>MQLWDINDHPYLNIKGRFQRDENGDEVWVVSAKRMWSLTQNEWLSADEVEIFDDPLYAGEPGFSAMIHDHEFAIHKHCTDVVVSGKARAYAKRPVEQMECRLLLDGHIDKTLVIHGQRDWIEHGGSITVSNPQSFIDCDIDYSHAIGGEDERNRIGGGVASSNKVLLTQRVPSVFYPKEDWDATSKKVRVAGFGPIPPFFKQRYQLAGTFDDNWLENRRPLLPVDFDRRYYQSAPLDQQCKGYLQGGERLMLSGFSHDDIFSFRLPREKYRASADFGDDQEFKDLELYTVFVDTEKGVVSLTYSAAFACQEKEHLLKSTSIQAVVENTNERGLNNEKLEHHHHHH[2x]

Type VI secretion systems (T6SSs) are dynamic protein nanomachines found in Gram-negative bacteria that deliver toxic effector proteins into target cells in a contact-dependent manner. Prior to secretion, many T6SS effector proteins require chaperones and/or accessory proteins for proper loading onto the structural components of the T6SS apparatus. Next, we present both genetic and biochemical evidence that PIPY domains require a cognate DUF2169 protein to form a functional T6SS spike complex with VgrG. Based on these findings, we propose a model whereby DUF2169 proteins function as molecular chaperones that maintain VgrG–PIPY spike complexes in a secretion-competent state prior to their export by the T6SS apparatus.

To circumvent this obstacle, we next screened a panel of DUF2169 proteins encoded by other Vibrio spp. that are closely related to V. parahaemolyticus and found that the DUF2169 protein from Vibrio xiamenensis, which shares 64% pairwise sequence identity with DUF2169 from V. parahaemolyticus, readily crystallized and we were able to solve its X-ray crystal structure to a resolution of 1.85 Å. The resulting electron density was of excellent quality, and we were able to model the majority of the 337 amino acid protein except for its three N-terminal and 12 C-terminal residues. The overall structure of V. xiamenensis DUF2169 reveals that its secondary structure is almost entirely comprised of β-strands arranged in three antiparallel β-sheets that form the core of the protein. These three β-sheets fold into two β-sandwiches that arise from the two shorter β-sheets stacking against the same face of the third, more elongated β-sheet. A search for structurally similar proteins in the Protein Data Bank using the DALI webserver indicates that the structure of DUF2169 is unique and therefore is considered a novel protein fold. Our structure also reveals that in its crystalline form, DUF2169 adopts a domain-swapped homodimeric arrangement with the swapped region (residues 195–232) consisting of a protruding loop that contains a short α-helix contributed by each protomer. The interface between the protomers is predominantly hydrophobic with several aromatic residues forming π-stacking interactions. In particular, Phe210 and Trp214 from one protomer π-stack with the equivalent residues from the other protomer. Collectively, these biophysical data support the conclusion that the domain-swapped dimer observed in our crystal structure is an artifact of crystal packing and that the protruding loop that facilitates this artifactual dimerization is highly dynamic and extends away from the core of the protein when it exists in its monomeric state in solution.> GSHMMKVEKEIKTNQDIDVVMTIFSDPAFTIPQIF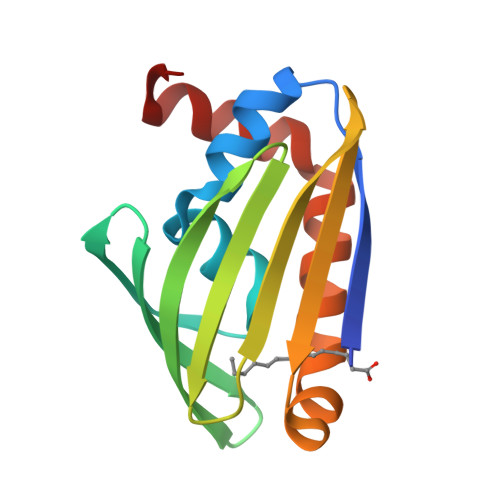PGIASIKCIEPEIFEAEGKFLAFSYKVKGRVYKGVDEVRIIYDSDRGNGILYIRKKDNNTLQIILEHDNKLTAFLGKPYVSSNLDRLAENIDEIIRLERIKRKI>[2x]HHHHHHNAKKSVYPLYYDSATVKKGLKSGTLFKGTLRILENHRSAFACMEDIPDFYVDGPIARNRAFHNDVVIVEPVMNNDSPTEKSNFLQNGVEKVKIKDHDDELGGAMEHLERLEIKSVASFKGDSRTRARVVAIEKRAEISKIVGILRAPGWSLKNVEYVSKKSSYAIFIPKDKRLPFITIHKNDLSDLSGENWIENILKHHDQLFSVEITRWSIYSRWPMGVLGEKLGNITDVEAYTNALLLENGISSSPFSDEVLNCLPPDDWIISHEEIKKRRDLRNELIITIDPETARDLDDAVSCRALDNGTYEVGVHIADVTHFVKPDSALDKEAASRATTVYLVQKAIPMLPPLLCERLCSLNPNVERLAFSVFWKLDSNGKEIGKRWFGKTVIKTCARLAYSEAQGVIEGKSWDDAVGKPIGGTHTPKD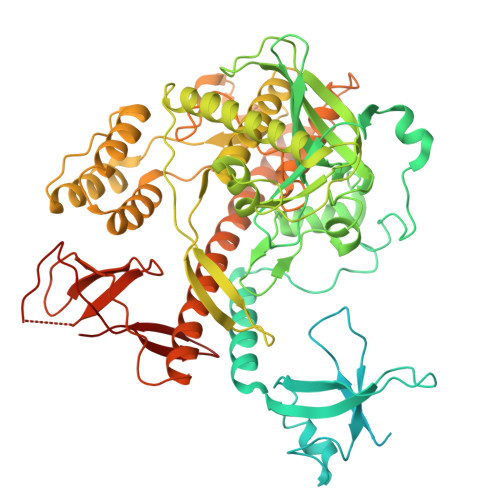VETSILTLCEISRKLRKDRFAKGAVEINSTELKFQLDEYGMPNKCEVYEQTDANHLIEEFMLLANRSVAEHISKNFSNNSLLRRHASPKEKQINEFCHFLKSMNFDFDASSSAAFNASMVRLRSTFNEELVELFENMAVRSLNRAEYFCTGDFGEKTDWHHYALSFNHYTHFTSPIRRYPDIIVHRLLERSLKNTSPGIDKKNCSLVAAHCNEKKEKSTTVQEDSQQLFLSVYIAEYCKKHDKKSMPVQAFATRISGNSIDVYISEYGISNRVDLSSDDRIKSFIVAPDDSSVKITLFDDSQKTIALTDRFQVYLYSDYSRTFFSIRCSLVSLN> NNFGA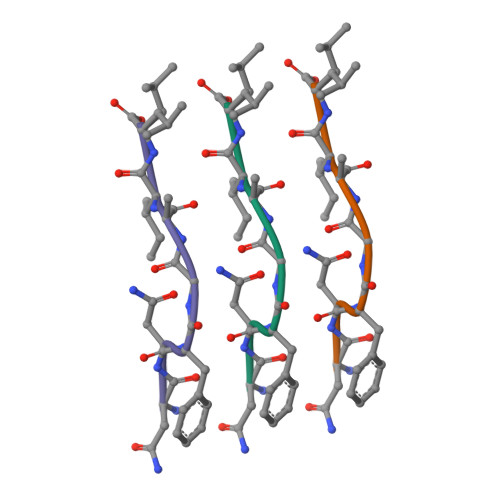IL> MNKRKINI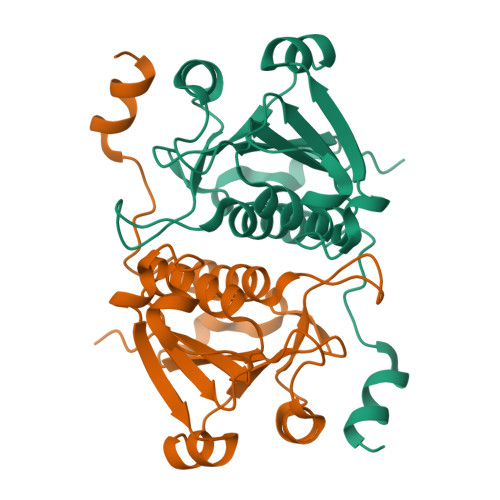VLYQPEIAQNVGAIMRTCVAINARLHIIEPLGFIFDDRHLSRSSANEYKYVDCIRYDDWNDFITKHQNITLFCLSRYGQKPISDFDFSKINDNVYLVFGKESTGIAKPILKEHYNTTFRIPMISETRSLNIANTVGIASYEVLRQWDYLDLVKYETQKGKDYILSERWKGIEEGHHHHHHG> MNKKTKLIHGGHTTDDYTGAVTTPIYQTSTYLQDDIGDLRQGYEYSRTANPTRSSVESVIAALENGKHGFAFSSGVAAISAVVMLLDKGDHIILNSDVYGGTYRALTKVFTRFGIEVDFVDTTHTDSIVQAIRPTTKMLFIETPSNPLLRVTDIKKSAEIAKEHGLISVVDNTFMTPYYQNPLDLGIDIVLHSATKYLGGHSDVVAGLVATSDDKLAERLAFISNSTGGILGPQDSYLLVRGIKTLGLRMEQINRSVIEIIKMLQAHPAVQQVFHPSIESHLNHDVHMAQADGHTGVIAFEVKNTESAKQLIKATSYYTLAESLGAVESLISVPALMTHASIPADIRAKEGITDGLVRISVGIEDTEDLVDDLKQ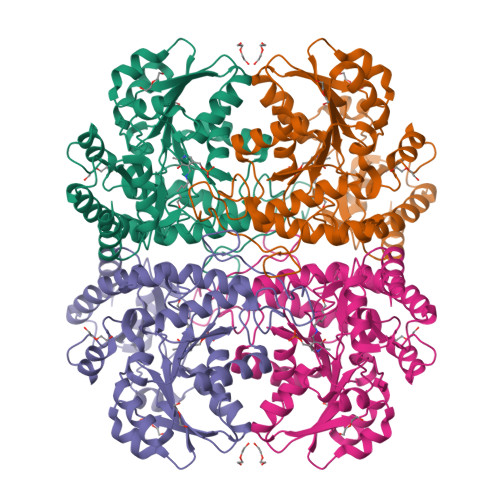ALDTL>MRVLALSAVFLVASIIGMPAVAKEWQENKSWNAHFTEHKSQGVVVLWNENKQQGFTNNLKRANQAFLAAST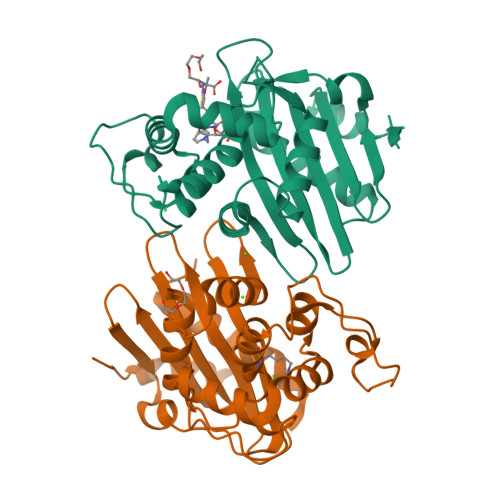FKIPNSLIALDLGVVKDEHQVFKWDGQTRDIATWNRDHNLITAMKYSVVPVYQEFARQIGEARMSKMLHAFDYGNEDISGNVDSFWLDGGIRISATEQISFLRKLYHNKLHVSERSQRIVKQAMLTEANGDYIIRAKTGYSTRIEPKIGWWVGWVELDDNVWFFAMNMDMPTSDGLGLRQAITKEVLKQEKIIP[4x]>GSRRASVGSHRFKVTNYMSPTFCDHCGSLLWGL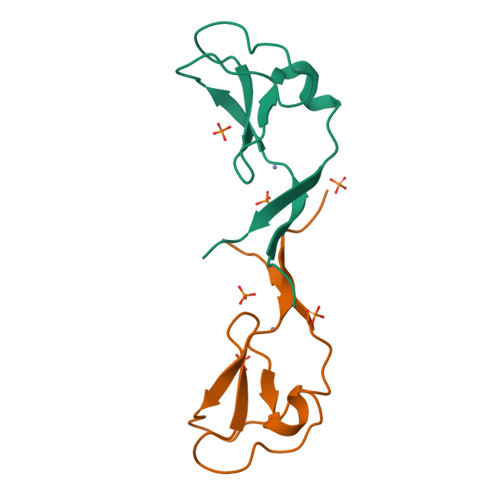VKQGLKCEDCGMNVHHKCREKVANLCEFIVTD[2x]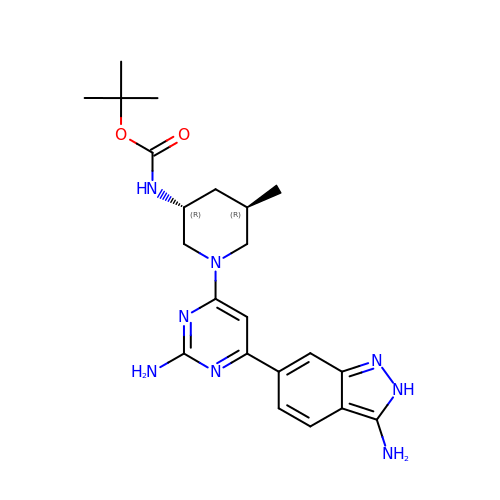tert-butyl {(3R,5R)-1-[2-amino-6-(3-amino-2H-indazol-6-yl)pyrimidin-4-yl]-5-methylpiperidin-3-yl}carbamate | C22 H30 N8 O2 | YEIVLMDWYXFKHN-TZMCWYRMSA-N>[2x]MTSITPVTLANCEDEPIHVPGAIQPHGALVTLRADGMVLAASENIQALLGFVASPGSYLTQEQVGPEVLRMLEEGLTGNGPWSNSVETRIGEHLFDVIGHSYKEVFYLEFEIRTADTLSITSFTLNAQRIIAQVQLHNDTASLLSNVTDELRRMTGYDRVMAYRFRHDDSGEVVAESRREDLESYLGQRYPASDIPAQARRLYIQNPIRLIADVAYTPMRVFPALNPETNESFDLSYSVLRSVSPIHCEYLTNMGVRASMSISI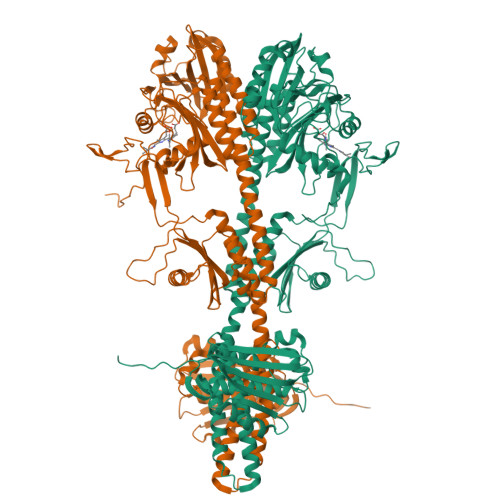VVGGKLWGLFSCHHMSPKLIPYPVRMSFQIFSQVCSAIVERLEQGRIAELLRVSTERRLALARRARDADDLFGALAHPDDGIAALIPCDGALVMLGGRTLSIRGDFERQAGNVLQRLQRDPERDIYHTDNWPQPSEDSPDGGDCCGVLAIRFHRQESGWIFWFRHEEVHRIRWGGKPEKLLTIGPSGPRLTPRGSFEAWEEVVRGHSTPWSETDLAIAEKLRLDLMELCLNHAAEVDRMRQRLIAVLGHDLRNPLQSISMAAALLSSSDTRTTELRQHISASSSRMERLVSQILDMSRLQSGIGLTVNPVDTDVSQLVRQIVCETDVAYPGLVIEIAIDPQVRAVVDPDRYAQVAANLLSNARHHGLPGRPVLVTLTRQGDEVCLSVLNETSGLSEAQLANLFEPFKRESADNQRNRNGLGIGLYISQAIAQAHQGRIDVDCRDDVITFCLRLPVRQAETGSSSLEHHHHHH> ITKVEAEN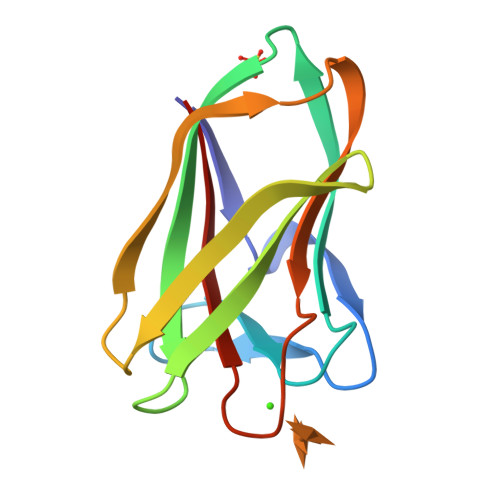MKIGGTYAGKISAPFDGVALYANADYVSYSQYFANSTHNISVRGASSNAGTAKVDLVIGGVTVGSFNFTGKTPTVQTLSNITHATGDQEIKLALTSDDGTWDAYVDFIEFSL> 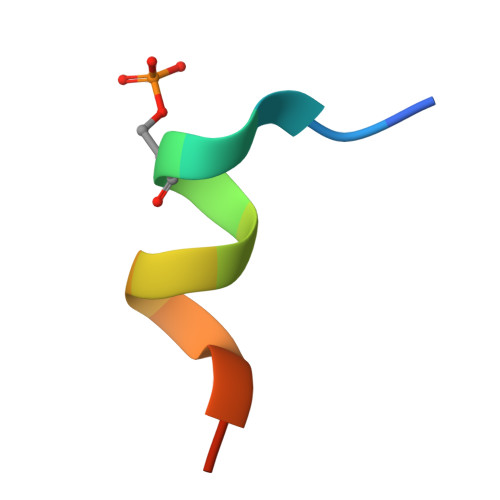IRSHSYLRAVSEVS> APITAYSQQTRGLLGCIITSLTGRDKNQVDGEVQVLSTATQSFLATCVNGVCWTVYHGAGSKTLAGPKGPITQMYTNVDQDLVGWPAPPGARSMTPCTCGSSD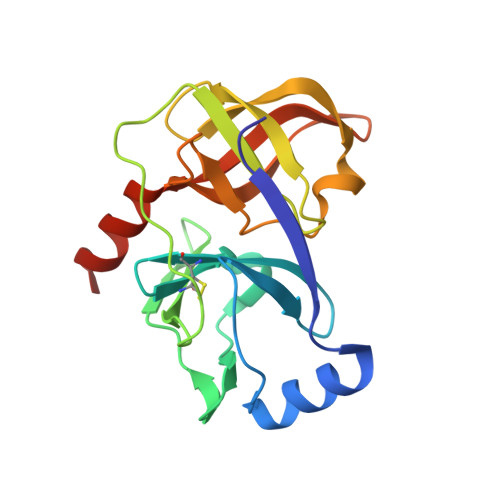LYLVTRHADVIPVRRRGDSRGSLLSPRPVSYLKGSSGGPLLCPSGHVVGIFRAAVCTRGVAKAVDFIPVESMETTMRASKKKK3-{2-[(5-AMINOPENTYL)AMINO]-2-OXOETHOXY}-5-({[1-(4-FLUOROPHENYL)ETHYL]AMINO}CARBONYL)PHENYL 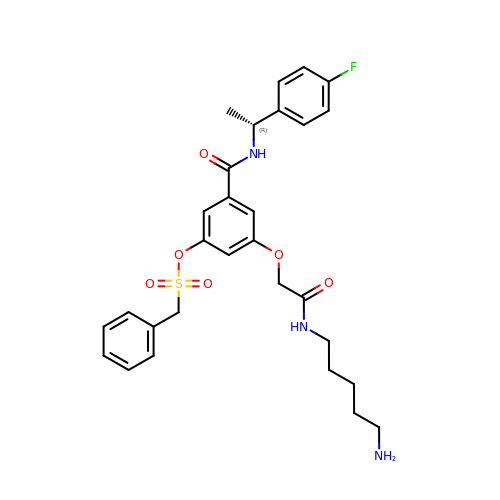PHENYLMETHANESULFONATE | C29 H34 F N3 O6 S | UUMRCVIXZFKZAU-OAQYLSRUSA-N(3~{S},6~{S})-3-[(4-hydroxyphenyl)methyl]-6-[(4-methoxyphenyl)methyl]piperazine-2,5-dione | C19 H20 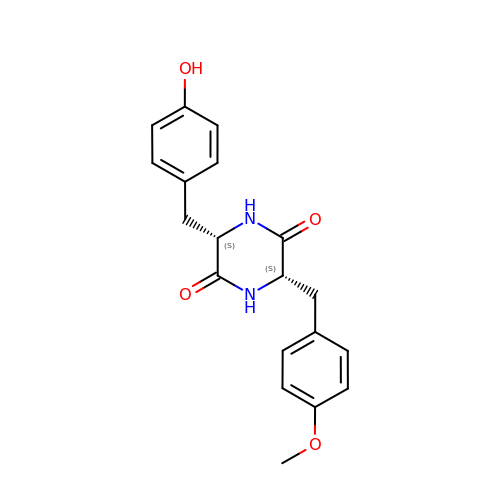N2 O4 | SXIBGFQFSYRUSU-IRXDYDNUSA-N>[2x]MSLNPALKFRDFIQVLKNEGDLIEIDTEVDPNLEVGAITRKAYENKLAAPLFNNLKQDPENIDPKNLFRILGCPGGLRGFGNDHARIALHLGLDSQTPMKEIIDFLVANRNPKKYIPPVLVPNDQSPHKKHHLTKEQIDLTKLPVPLLHHGDGGKFIQTYGMWVLQTPDKSWTNWSIARGMVHDSKSITGLVINPQHVKQVSDAWVAAGKGDKIPFALCFGVPPAAILVSSMPIPDGATEAEYIGGLCNQAVPVVKCETNDLEVPADCEMVFEGYLDRDTLVREGPFGEMHGYCFPKDHHTQPLYRVNHISYRDQAIMPISNPGLCTDETHTLIGGLVSAETKYLISQHPVLSKIVEDVFTPYEAQALWLAVKINTHELVKLKTNAKELSNLVGDFLFRSKECYKVCSILHEIILVGDDIDIFDFKQLIWAYTTRHTPVQDQLYFDDVKPFALAPFASQGPLIKTRQGGKCVTTCIFPKQFTDPDFEFVTCNFNGYPEEV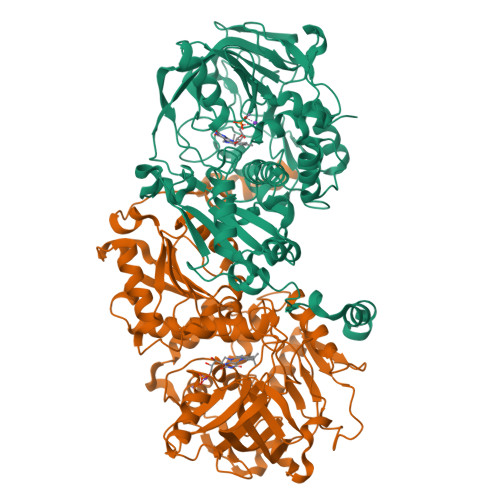KNKISQNWDKYYK> SHMRSAQVYRWQIPMDAGVVLRDRRLKTRDGLYVCLREGEREGWGEISPLPGFSQETWEEAQSVLLAWVNNWLAGDCELPQMPSVAFGVSCALAELTDTLPQAANYRAAPLCNGDPDDLILKLADMPGEKVAKVRVGLYEA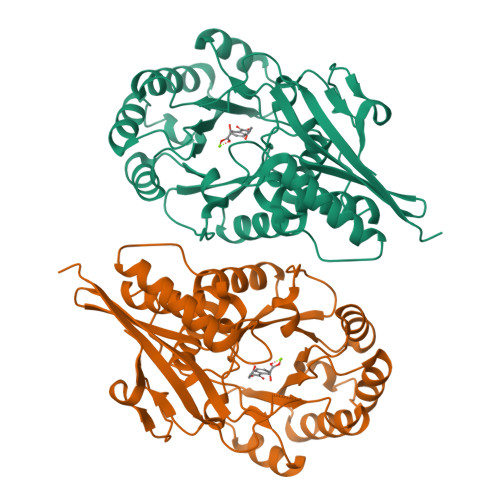VRDGMVVNLLLEAIPDLHLRLDANRAWTPLKGQQFAKYVNPDYRDRIAFLEEPCKTRDDSRAFARETGIAIAWDESLREPDFAFVAEEGVRAVVIKPTLTGSLEKVREQVQAAHALGLTAVISSSIESSLGLTQLARIAAWLTPDTIPGLDTLDLMQAQQVRRWPGSTLPVVEVDALERLL> MQQLNENKIIKLLRDNIPKLQLIYLFGSYSQGTQHRNSDIDIAVLAADTLDNIARWELAQKLASALDSDVDLVDLRSASTVLCQQVVTQGKQLWGTQQDDELFAVKTISMYQHLQAERQAIIDDVMANTAAKAHRGES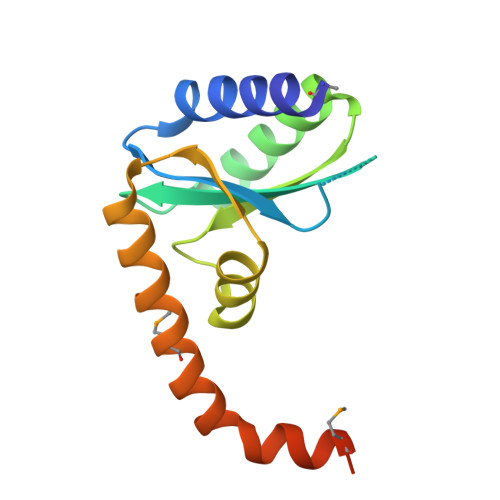L> MSE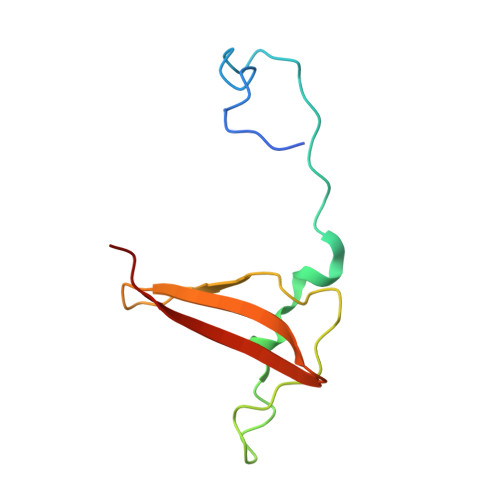SEQYSTEIPAFLTSNTLQELKLPKPPSLPPHLEKCILNSNTAYKEDQSVLPNPNHVLLNHLAAANTQLGVLALSATTRYHRKYVTTAMFKNFDV>[8x]ADPAPTS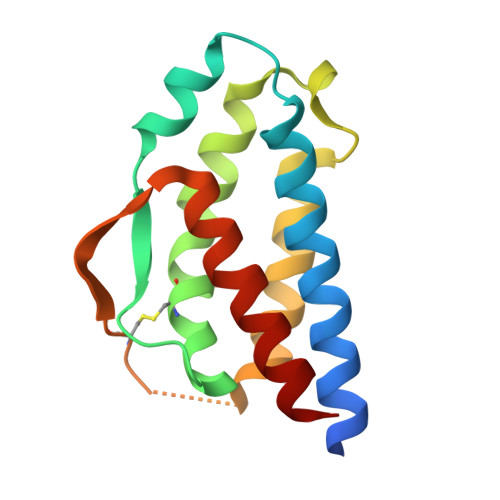SSTKKTQLQLEHLLLDLQMILNGINNYKNPKLTRMLTFKFYMPKKATELKHLQCLEEELKPLEEVLNLAHSKNFHFDPRDVVSNINVFVLELKGSETTFMCEYADETATIVEFLNRWITFCQSIISTLT> MTEAIDWDQMNNQVIKEFRETGGKAGGLFEGSPLVLVHHTGAKSGKQRIAPLVPLLDGDRIYIFGSKGGADSHPDWYHNLVANPDTVVELGTETFPVKARVLTGAERDEIY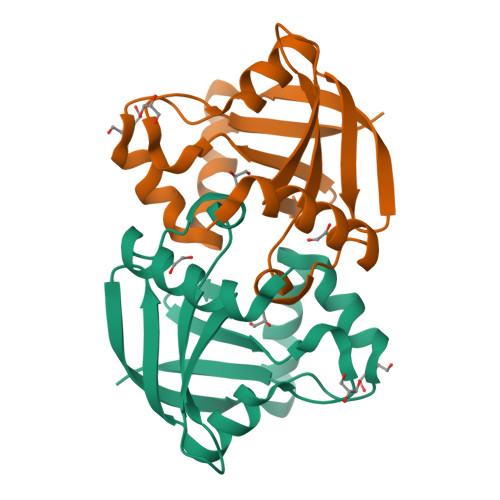AKQVAVAPQFGDYQRKTTRVIPVVELQRV>GMTVRDENYFTEKYGLTRTHSDVLAAAKVVAPGRTLDLGCGNGRNSLYLAANGYDVTAWDKNPASMANLERIKAAEGLDNLQTDLVDLNTLTFDGEYDFILSTVVMMFLEAQTIPGLIANMQRCTKPGGYNLIVAAMDTPDFPCTVGFPFAFKEGELRRYYEGWD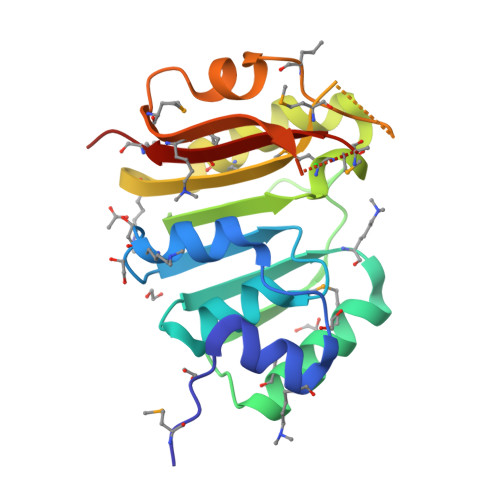MLKYNEDVGELHRTDENGNRIKLRFATMLARKTA[2x]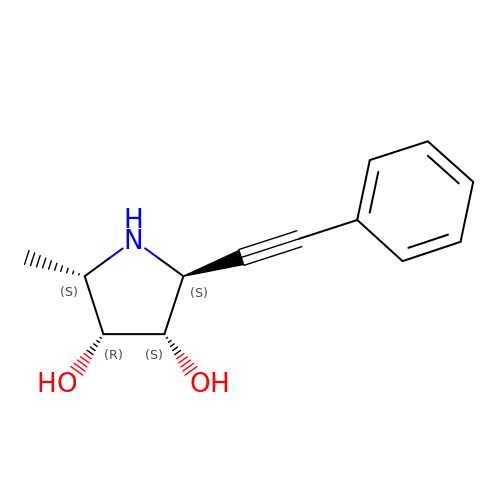(2S,3R,4S,5S)-2-methyl-5-(phenylethynyl)pyrrolidine-3,4-diol | C13 H15 N O2 | RPIQJUPODSDSQH-SYEHKZFSSA-N> IVGGSNAKEGAWPWVVGLYYGGRLLCGASLVSSDWLVSAAACVYGRNLEPSKWTAILGLHMKSNLTSPQTVPRLIDEIVINPHYNRRRKDNAIAMMHLEFKVNYTDYIQPICLPEENQVFPPGRNCSIAGWGTVVYQGT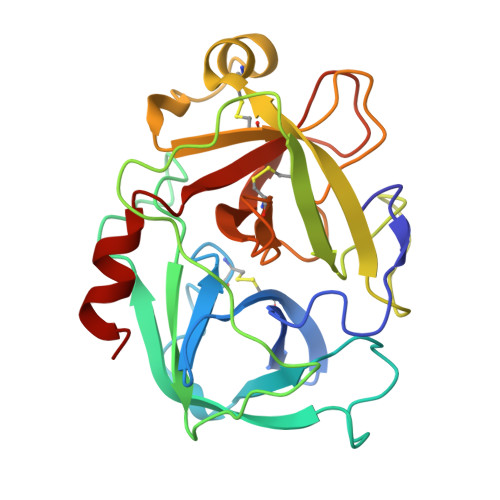TANILQEADVPLLSNERCQQQMPEYNITENMICAGYEEGGIDSCQGDAGGPLMCQENNRWFLAGVTSFGYKCALPNRPGVYARVSRFTEWIQSFLH>[2x]HHHHHHVGCSVDFSKKETRCGTGVFVYNDVEAWRDRYKYHPDSPRRLAAAVKQAWEDGICGISSVSRMENIMWRSVEGELNAILEENGVQLTVVVGSVKNPMWRGPQRLPVPVNELPHGWKAWGKSYFVRAAKTNNSFVVDGDTLKECPLKHRAWNSFLVEDHGFGVFHTSVWLKVREDYSLECDPAVIGTAVKGKEAVHSD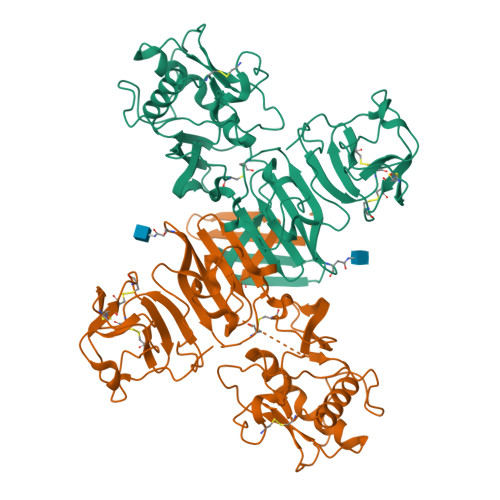LGYWIESEKNDTWRLKRAHLIEMKTCEWPKSHTLWTDGIEESDLIIPKSLAGPLSHHNTREGYRTQMKGPWHSEELEIRFEECPGTKVHVEETCGTRGPSLRSTTASGRVIEEWCCRECTMPPLSFRAKDGCWYGMEIRPRKEPESNLVRSMVTA>[2x]MFSPVVVSVVFTIAFCNASPARDSFGCSNSGITDSDRQAFLDFHNNARRRVAKGLEDSNSGKLNPAKNMYKLSWDCAMEQQLQDAIQSCPSGFAGIQGVAQNTMSWSSSGGYPDPSVKIEPTLSGWWSGAKKNGVGPDNKYTGGGLFAFSNMVYSETTKLGCAYKVCGTKLAVSCIY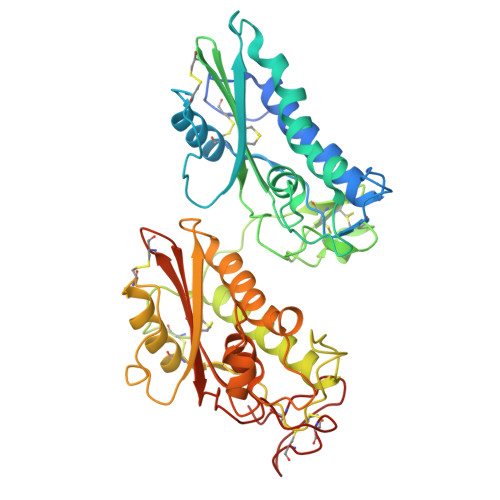NGVGYITNQPMWETGQACQTGADCSTYKNSGCEDGLCTKGPDVPETNQQCPSNTGMTDSVRDTFLSVHNEFRSSVARGLEPDALGGNAPKAAKMLKMVYDCEVEASAIRHGNKCVYQHSHGEDRPGLGENIYKTSVLKFDKNKAAKQASQLWWNELKEYGVGPSNVLTTALWNRPNMQIGHYTQMAWDTTYKLGCAVVFCNDFTFGVCQYGPGGNYMGHVIYTMGQPCSQCSPGATCSVTEGLCSAP> SAGKFIVIFKNDVSEDKIRETKDEVIAEGGTITNEYNMPGMKGFAG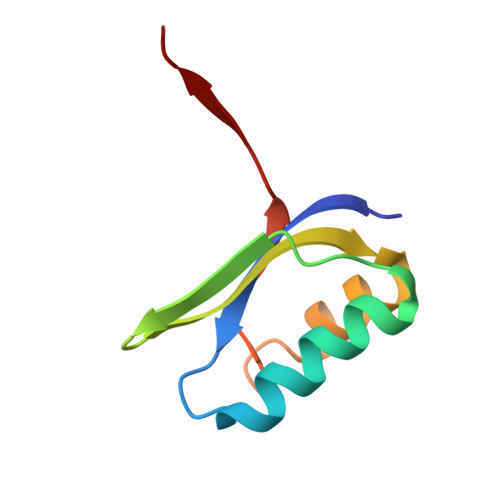ELTPQSLTKFQGLQGDLIDSIEEDHVAHAY> TADELVFFVNGKKVVEKNADPETTLLAYLRRKLGLRGTKLGCGEGGCGACTVMLSKYDRLQDKIIHFSANACLAP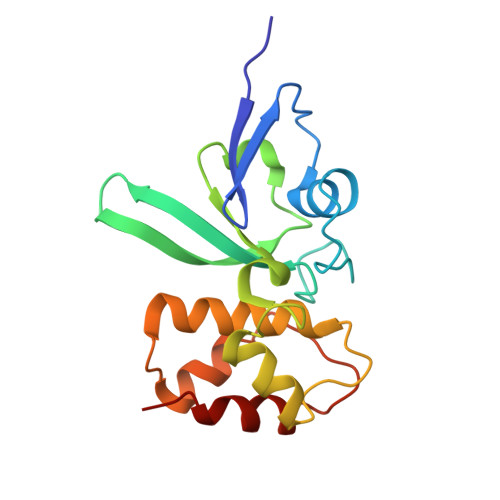ICTLHHVAVTTVEGIGSTKTRLHPVQERIAKSHGSQCGFCTPGIVMSMYTLLRNQPEPTVEEIEDAFQGNLCRCTGYRPILQGFRTFAK>[8x]MDWSHPQFEKKKKAEWPRKLRSQEWYGGTSRDVIYHRGWLKNQGYPHDLFDGRPVIGILNTWSDMTPCNGHLRELAEKVKAGVWEAGGFPLEVPVFSASENTFRPTAMMYRNLAALAVEEAIRGQPMDGCVLLVGCDKTTPSLLMGAASCDLPSIVVTGGPMLNGYFRGERVGSGTHLWKFSEMVKAGEMTQAEFLEAEASMSRSSGTCNTMGTASTMASMAEALGMALSGNAAIPGVDSRRKVMAQLTGRRIVQMV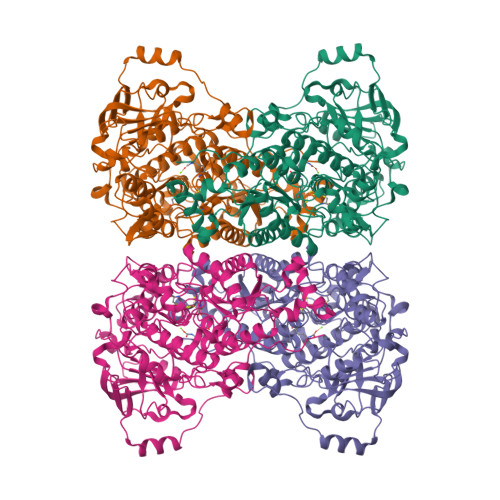KDDLKPSEIMTKQAFENAIRTNAAIGGSTNAVIHLLAIAGRVGIDLSLDDWDRCGRDVPTIVNLMPSGKYLMEEFFYAGGLPVVLKRLGEAGLLHKDALTVSGETVWDEVKDVVNWNEDVILPAEKALTSSGGIVVLRGNLAPKGAVLKPSAASPHLLVHKGRAVVFEDIDDYKAKINDDNLDIDENCIMVMKNCGPKGYPGMAEVGNMGLPPKVLKKGILDMVRISDARMSGTAYGTVVLHTSPEAAVGGPLAVVKNGDMIELDVPNRRLHLDISDEELARRLAEWQPNHDLPTSGYAFLHQQHVEGADTGADLDFLKGCRGNAVGKDSH> SMYAIRKIQFFYGPTDKKSYVGEEAGGRRELFKTRAEAQARIEDLEEGVYYLAHNESGRPDYKIVWVRGE;>TIEKRYDFVFLFDVQDGNPNGDPDAGNLPRIDPQTGEGLVTDVCLKRKVRNFIQMTQNDEHHDIFIREKGILNNLIDEAHEQENVKGKEKGEKTEAARQYMCSRYYDIRTFGAVMTTGKNAGQVRGPVQLTFSRSIDPIMTLEHSITRMAVTNEKDASETGDNRTMGRKFTVPYGLYRCHGFISTHFAKQTGFSENDLELFWQALVNMFDHDHSAARGQMNARGLYVFEHSNNLGDAPADSLFKRIQVVKKDGVEVVRSFDDYLVSVDDKNLEETKLLRKLGG[7x];>[4x]GLDRNRQDIGYVLGRLFAVLEKIQAEANPGLNATIADRYFGSASSTPIAVFGTLMRLLPHHLNKLEFEGRAVQLQWEIRQILEHCQRFPNHLNLEQQGLFAIGYYHETQFLFTKDALKNLFNEA;> MILHALTQYYQRKAESAQKGICLVTGKAAPIARLHNAVKGVNAKPAPFASVNLSAFESYGKEQGFAFPIGEQAMFEYTTALNTLLAGENRFRIGDVTTVCWGAKRTPLEESLASMINGGGKDKPDEHIDAVKTLYKSLYNGQYQKPDGKEKFY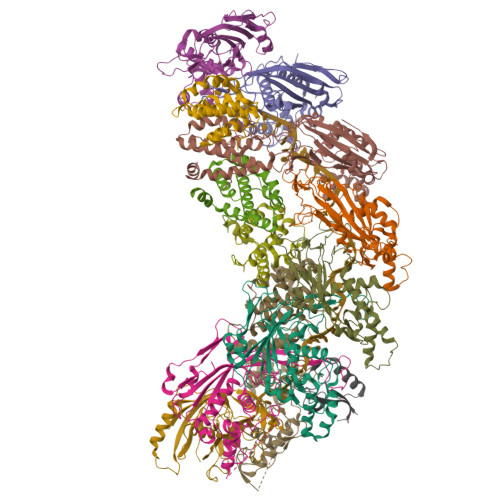LLGLSPNSARIVVRFWHETTVAALSESIAAWYDDLQMVRGENSPYPEYMPLPRLLGNLVLDGKMENLPSDLIAQITDAALNNRVLPVSLLQAALRRNKAEQKITYGRASLLKAYINRAIRAGRLKNMKELTMGLDRNRQDIGYVLGRLFAVLEKIQAEANPGLNATIADRYFGSASSTPIAVFGTLMRLLPHHLNKLEFEGRAVQLQWEIRQILEHCQRFPNHLNLEQQGLFAIGYYHETQFLFTKDALKNLFNEA;> RFILEISGDLACFTRSELKVERVSYPVITPAAARNILMAILWKPAIRWKVLKIEILKPIQWTNIRRNEVGTKMSERSGSLYIEDNRQQRASMLLKDVAYRIHADFDMTSEAGESDNYVKFAEMFKRRAKKGQYFHQPYLGCREFPCDFRLLEKAEDGLPLEDITQDFGFMLYDMDFSKSDPRDSNNAEPMFYQCKAVNGVITVPP> QVAEDCMGLLQLLSNGTVLRSESIDLITQQIPFKNNQTVLFKDSIYHKPNNLHLRLYKPISASNRTALPVVVFFHGGGFCFGSRSWPHFHNFCLTLASSLNALVVSPDYRLAPEHRLPAAFEDAEAVLTWLW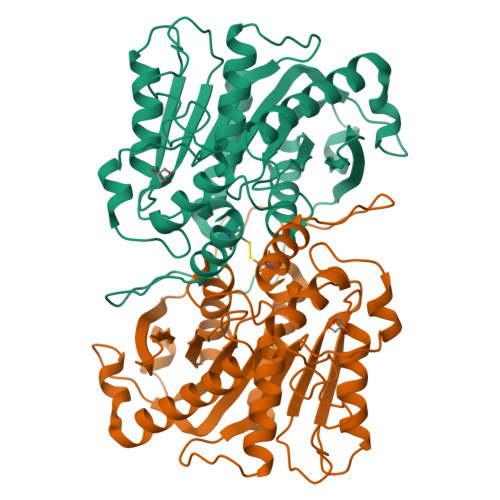DQAVSDGVNHWFEDGTDVDFDRVFVVGDSSGGNIAHQLAVRFGSGSIELTPVRVRGYVLMGPFFGGEERTNSENGPSEALLSLDLLDKFWRLSLPNGATRDHHMANPFGPTSPTLESISLEPMLVIVGGSQLLRDRAKEYAYKLKKMGGKRVDYIEFENKEHGFYSNYPSSEAAEQVLRIIGDFMNNLS> RQLNVNAK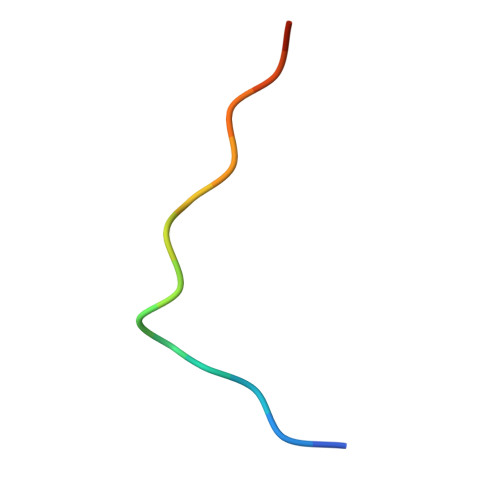PFVPNVH>[4x]MQHHWKELIAVDRYTVQSRGVLQEVDRKVLTLLYQPLIGCRALALYMT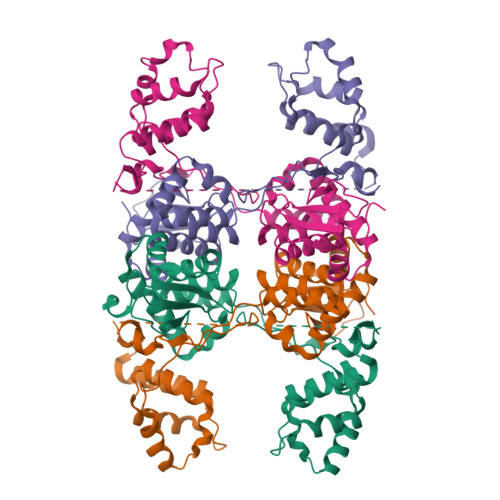LWGELELLDGQEATHHRLMALMQCGLPDIYSERLKLEGIGLLDTYVHAKEADEPKLFLYELRPPLAPDQFFRDEMLSVFLRRQVGRHLFIQLSNFFARPSIDETKFTQVTRSFSDVFSAVPAEQIVAGLSEEAGPELLEGKDHIRRDEASYVLDDGVFDFELFFAGLSKQLVPRRAVTAKVKEAIKKLAFLYGIPPLEMQKLVLGVIDPAYHIDIDALRRAAREWYELEHGGVEPRLVERVQPLAYRTMENI> PADRLKALVDAAVQPVMKANDIPGLAVAISLKGEPHYFSYGLASKEDGRRVTPETLFEIGSVSKTFTATLAGYALTQDKMRLDDRASQHWPA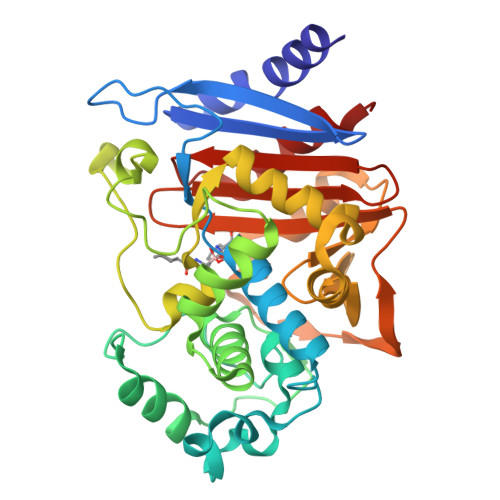LQGSRFDGISLLDLATYTAGGLPLQFPDSVQKDQAQIRDYYRQWQPTYAPGSQRLYSNPSIGLFGYLAARSLGQPFERLMEQQVFPALGLEQTHLDVPEAALAQYAQGYGKDDRPLRVGPGPLDAEGYGVKTSAADLLRFVDANLHPERLDRPWAQALDATHRGYYKVGDMTQGLGWEAYDWPISLKRLQAGNSTPMALQPHRIARLPAPQALEGQRLLNKTGSTNGFGAYVAFVPGRDLGLVILANRNYPNAERVKIAYAILSGL>[2x]MAITEFDTSLPSIRQLQNLIKQAAPVEIKLVTGDAITGRVLWQD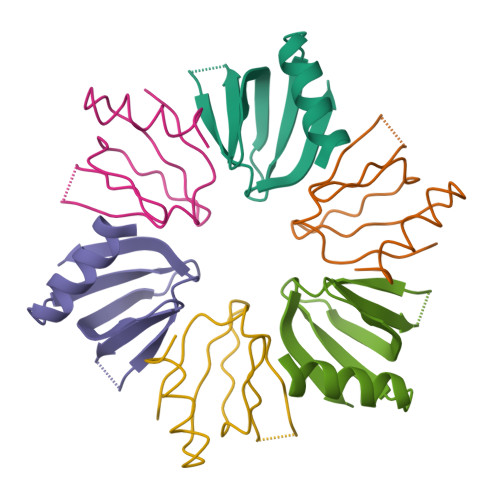PTCVCIADENSRQTTIWKQAIAYLQPKG> DCTSLNRLLVKRQWAEAYGEGTNRELLGNRIWEDLFANMPDARGLFSRVNGNDIDSSEFQAHSLRVLGGLDMCVASLDDVPVLN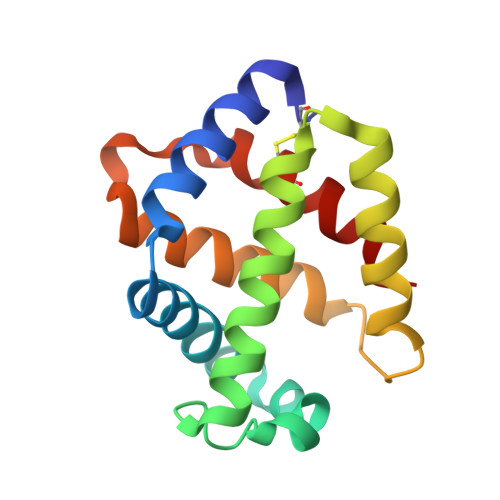ALLARLNSQHDSRGIPAAGYPAFVASAISAVRATVGARSFDNDAWNSCMNQIVSGISG>[4x]DLADRFAELERRYDARLGVYVPATGTTA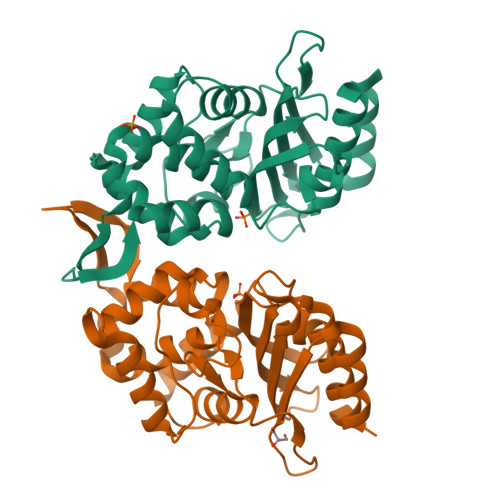AIEYRADERFAFCSTFKAPLVAAVLHQNPLTHLDKLITYTSDDIRSISTVAQQHVQTGMTIGQLCDAAIRYSDGTAANLLLADLGGPGGGTAAFTGYLRSLGDTVSRLDAEEPELNRDPPGDERDTTTPHAIALVLQQLVLGNALPPDKRALLTDWMARNTTGAKRIRAGFPADWKVIDKTGTGDYGRANDIAVVWSPTGVPYVVAVMSDRAGGGYDAEPREALLAEAATCVAGVLA>GMKTRLEQVLERYLNGREVAVWGVPTRRLLRALKPFKFHTADRVDPQYHYVVAVTDDDLTDFLSDEQSKSFQYANDYLTFDDEGGELPFERMCFNVPVGRQTYFGDGVVGACENGYIKSIGQFTSINGTAEIHANHQLNMTFVSDDIQNFFNEESMAVFQEKLRKDPKHPYAYSKEPMTIGSDVYIG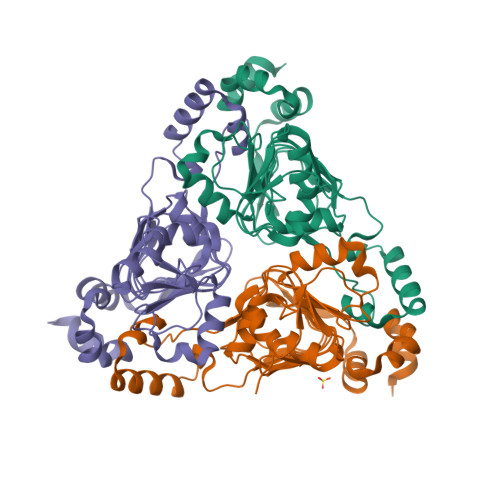AHAFINASTVTSIGDGAIIGSGAVVLENVPPFAVVVGVPARIKRYRFSKEMIETLLRVKWWDWSIEEINENVDALISPELFMKKYGSL[3x]>GHMAEVLVVTSKVKKLIKEKGQMNTSAETIDVLSKAIEQLCLKGVESAKADGRKTVMARDIVIDHL[2x]

In this study, we present crystal structures and biochemical characterization of the free and DNA-bound forms of the histone homolog HBb from the predatory Gram-negative bacterium Bdellovibrio bacteriovorus. Our findings demonstrate that the single histone fold protein HBb forms a homodimer that has the ability to bind and bend DNA. Furthermore, we establish that HBb is essential for maintaining bacterial viability. Building on this, by employing various biophysical and biochemical approaches, we further substantiated the ability of HBb to bind and compact DNA by bending in a sequence-independent manner.

Similar to its free form, HBb successfully crystallized in complex with a randomized 20 bp DNA fragment (20 bp-GC50) within a few days, yielding the two distinct crystal forms HBb-DNA_1 and HBb-DNA_2. These could be processed to a resolution of 1.95 Å (HBb-DNA_1) and 1.85 Å (HBb-DNA_2), and solved by molecular replacement using the free form of HBb as a search model. Additionally, clear electron density for short DNA fragments was apparent in both structures, albeit in different positions. For HBb-DNA_1, the asymmetric unit contains a 5 bp dsDNA fragment, which forms an infinite dsDNA helix throughout the crystal via crystallographic symmetry. Both monomers of the HBb dimer interact with the minor groove of this DNA. Specifically, residues K12 in helix α1, T23 and S24 in loop l1, and A25 in helix α2 of one monomer, as well as K52 and T53 in loop l2 and R57 in helix α3 of the other monomer, form an interaction network with the phosphate groups of the DNA backbone through their side chains and backbones. The superposition of the HBb-DNA_1 and HBb-DNA_2 structures illustrates the location of the combined HBb-DNA binding interfaces, resembling histone-DNA complexes found in eukaryotes and archaea. The engagement of these interfaces suggests that the DNA undergoes bending upon binding with the HBb dimers. For the starting structure, we combined the HBb-DNA_1 and HBb-DNA_2 crystal structures to create a complete DNA molecule bent around the HBb dimer.>QSVDIHKDQIIFSEGDAGDCAYIIEKGRVLIYLTKDKEEIPLTILGEGEIFGEMALIDNQNRSASVRALEDVRLAIVTKQQVLERVSTADKVVQLLMRVLLKRLRRKNIGGPGGSRISEVEFDNSGAGDDGTQSALDQIKLENQIFQAFQNKEFELFYQPIVNLKNKTITGCEALLRWNSPQHGLVSPNLFIDIIENSSMVIPIGHWIINQALKDLRTIQDQLRLNKKERMADDFMMSINISGRQFTHSDFVNNLEDLREKHDLHTQNIKLEMTERIMMDGAIAIDALNQCRSLGYAISIDDFGTGFSGLQYLTQMPISFLKIDRSFVMKILSDPKSKAVVSSIIHLAHAMDIEVIAEGIEHHEEALVLETLGARFGQGYLFSKPVDLGRFLKLIKL[2x]

Herein, we provide high‐resolution structures for an EAL enzyme Bd1971, from the predatory bacterium Bdellovibrio bacteriovorus, which is controlled by a second signaling nucleotide, cAMP. The Bd1971 domain architecture is predicted to consist of an N‐terminal cNMP sensory domain (cyclic nucleotide monophosphate, postulated to bind cAMP or cGMP), a middle linker region, and C‐terminal catalytic EAL barrel. We reveal that regulation of c‐di‐GMP hydrolysis arises from a domain‐swapping of the “regular” cNMP fold, which undergoes significant rearrangements upon binding of stimulus, communicating a series of conformational changes over 40 Å to license a productive state at the EAL dimer interface. C‐di‐GMP turnover was increased ~8‐fold in the presence of cAMP or cGMP, further supporting the proposal that cNMPs are activators of Bd1971.

The crystal structure of full‐length Bd1971 was solved with both cAMP and cGMP ligands, to resolutions of 2.63 and 2.46 Å, respectively. These two co‐crystal structures are effectively identical other than small differences at the ligand binding pocket that are discussed later. The full‐length cAMP‐bound form reveals the sensory N‐terminus to be a domain‐swapped variant of the cNMP/CRP family, which in the cAMP‐activated state holds the C‐terminal EAL enzyme in a phosphodiesterase‐active conformation. Bd1971 forms a butterfly shaped dimer measuring 90 Å tall, 90 Å wide (at larger EAL domain) and 40 Å deep. The central twofold axis acts to situate an EAL domain dimer (residues 158–402) over a cNMP sensor dimer (6–111). Bd1971 dimerizes around a long helix (residues 340–357) and a shorter helix (315–321, referred to as the compound helix in BlrP1 or repressor helix in MorA; Phippen et al, 2014) that follows the catalytic aspartate pair (Asp306/307), and can thus be assigned to the “open” grouping that correlates with active enzymes. The dimerization interface we observe is centered around Ser348 and places Asp306 and Asp307 in a productive orientation, similar to that observed in other (presumed active) EAL dimers. Superimposition using the cAMP ligand reveals many shared residues/structural features between Bd1971 and CRP including the classical base capping residue (Bd1971 Arg108: CRP Arg123), phosphate cradle (Arg67/Ser68: Arg82/Ser83), and ribose‐coordinating group (Glu58:Glu72). Due to the relative C‐helix swapping, the hydrophobic base capping residues (Arg108 and Leu109) are contributed from the opposing monomer in Bd1971 and the same monomer in CRP. Importantly, the linker helix (residues 136–157) is central to the productive full‐length bound form, contacting three separate domains—both cNMP sensors (one chain via the N‐terminal end of the C‐helix, the other chain via the outward face of the β‐sandwich), and the EAL domain (at the αββα start of the barrel).> GSHMQNNSAKQSWLLRLFESKLFDISMAISYLYNSKEPGVQAYIGNRLFCFRNEDVDFYLPQLLNMYIHMDEDVGDAIKPYIVHRCRQSINFSLQCALLLGAYSSDMHISTQRHSRGTKLRKLILSDELKPANLKRTAANPKVENEDEPVRLAPEREFIKSLMAIGKRLATLPTKEQKTQRLISELSLLNHKLPARVWLPTAGFDHHVVRVPHTQAVVLNSKDKAPYLIYVEVLECENFDTTSVPARIPENRRDPEDPSAVALKEPWQEKVRRIREGSPYGHLPNWRLLSVIVKCGDDLRQELLAFQVLKQLQSIWEQERVPLWIKPYKILVISADSGMIEPVVNAVSIHQVKKQSQLSLLDYFLQEHGSYTTEAFLSAQRNFVQSCAGYCLVCYLLQVKDRHNGNILLDAEGHIIHIDFGFILSSSPRNLGFETSAFKLTTEFVDVMGGLDGDMFNYYKMLMLQGLIAARKHMDKVVQIVEIMQQGSQLPCFHGSSTIRNLKERFHMSMTEEQLQLLVEQMVDGSMRS;> GSHMGTRDDEYDYLFKVVLIGDSGVGKSNLLSRFTRNEFNLESKSTIGVEFATRSIQVDGKTIKAQIWDTAGLERYRAITSAYYRGAVGALLVYDIAKHLTYENVERWLKELRDHADSNIVIMLVGNKSDLRHLRAVPTDEARAFAEKNGLSFIETSALDSTNVEAAFQTILTEIYRIVSQKQMSDRRENDMSPSNNVVPIHVPPTTENKPKVQCCQN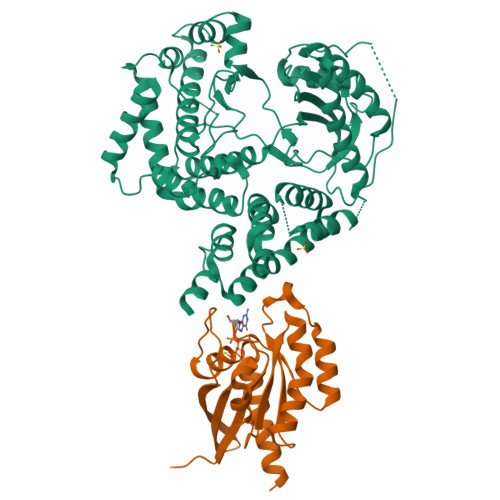I> GPGSMAAGTQVIANSGHDDMIHDAVLDYYGRRLATCSSDRTIKIFEIEGETQRLTETLKGHDGAVWCVSWAHPKYGNILASAGYDGKVLIWRELNGAWQRIFDFALHKASVNVVSWSPHEAGCLLACASSDGNVSVLEFRDNSWEHSIFHAHGLGVNSVSWAPATSPGSIVSSKPGPKSTGNRRFVTGGSDNALKIWAYDPATNTYKLEREPLTGHTDWVRDVAWSPTVLQKSYIASASEDRTVRIWTSDPANPLQWNCKVLNFDAAVWRVSWSLSGNVLAASGGDNKVTLWKENLKGEWECVKTIEEGGGGSGGGGQAKGPTQPEQASPAKGFVKWPYQQRPKIDQQEGPSIPRTNWGPNGLLVT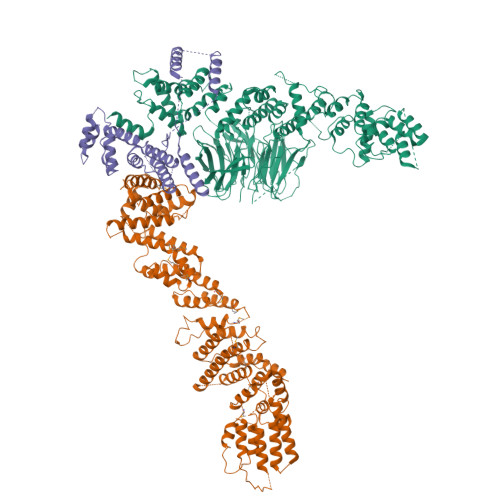THHGEPSLQPADGTLAASEESVGSPENLARLQRYIDSVSFKEGQPIASPEFRELAQGDPSWELASLLFDDNGYGLPAFWRQLVSEATDRALAQEPGLEEKAIICLAGNRVADACGYLLAAGNFRLATLVSGIGMQDGDMKAQLKDWRESNVLAEFSQPVRAIYELLAGNAGVCAGVKNVPIENRVDSFTISQRFGLDWMRSFGLRLFYTTGATANVAEAVRSFQADIEQDKEPEPDSALWSLLKAFANQEFDWSDTRLGWLLTKAIYATGKVSFGQDAAEKLDKASLAYASALTAQSQWVPATFVLLQLSDAASREAAVRDHLGRHARRIGSPRNPNSAFSSLRKFGVPETWIWEAKALDFRARGDSQQEFLALVWAQNYSEANQAFVHRVGPDLVIARDFRRLFRFAQLLFKVKGKLQDWDRGAAVYLLYPMARLQGKQHGLDKFDHQLFDGLVALRGQTHGDIRQEAAIADMAEDLIRCRGGDPRLFGLLPEDVRSKYMRAQALEVIC;> GPGSEFELMWLDMPSTAETGADQPAAGEVSDLLMLATPAATERVRREAEDIFRASSFRAGGAARRSEYRYAALAKDAYQQMGTAPVTEPPQVILGTEDLLSRLYDEGVGEAEDEQKMDDTLATAAAQLAALWREHVDELPRPTEDHAAEIGPGPHATPFEKANYLANLALQIHHTRYEEGGLIRAEPLPQTLFRWLNEYHDMYGSQVDDILRHRPSPACHSLFWQAVFIALLRGKVGDAARLLDQAGWGHVRRGQRGEYAYVGQALENVQRAVDETIAVLESCPGFDGNWEIWSSDWTLFRVRARGLLEHLRRFAEGKDSAFGASAFSASAASAQSRQSMAGLARRAESQVPWEIYENLNIVFDIVLGQQGAILEAAQDWLEATVGLFGWWDERASRTEKPLSTSQSLSRSQALVLASAPANSESYLDRLARAFHTAVESDFHFNSQNAVEIGMACVFEDNIKGVIGLLRGWSLPIAAAVAEIASLGKWLPPHRPSGVYGLEDLDMDDLEVLGMDPGAPDEVDGIKDSTLVQYAQALADYEGLSSVQDRSGTSKDGWELSISVLGRMDSPERSEEMVRDLVEHLVQQLHVDSNATVDRLWFLLNELGMIEFAEDTTETYGDILARDSHRYGEAMWYYALAHRPNKVREVMNLLTSYSLIQSTAFPPANDLDDYLYKLLNDRKNTLEQCASQDMEAAELLGKMLSGYASLRQFYDIRDNEDALPHATPLSRRKQAATALISVIASSDDNIRGGLYDQTRDGIVSEDFLLALLGEALVFVSDPDNTNVHHGQLATPVITLDQIDVLLKAIEDLQAVGSRVYNACDEFLQLVLASAPGGLKGSTPADLLKKSAGPGPGGSGNAMLAGSSLVASQLQRSLSGTGGGLGKVAVKRRGWDWRSEVTAKTKGEDIMRRLRLGLAKDLAGLWLAEADEMVW;> GPGSEFELMQGGSSTNHETAGLRTEMLSRLFTAATSISHFEEAHSALLSMDDEAMQKSYLRRLVEKMCETGQSSELITLPFSGLQTKVDDILVEKCRATRDVLNGVPYHQILYAWRINHNDYRGGAAILLDRLQKLRRAGEGDKVIANEHGNEDALDTQVTRQYLLLINALSCVPPQEAYILEDVLPGDGRGGDDADGDRNGGKAGDDLEADIDELEKKLDVEGGADAAKGDEMAAEEDAALIEKMKRFSTRNGQNLPARRLLMLADLRKQYQQELDRIVAIQNNQFGFGAEDDLMDLAGGSGHHHHHHHHHH> TRSK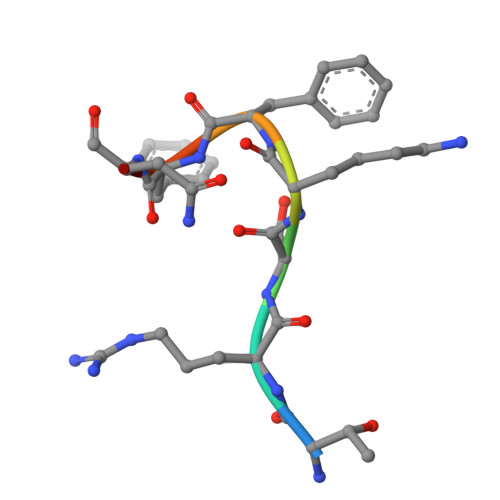FFNK N-(dimethoxyphosphoryl)-beta-D-glucopyranosylamine | C8 H18 N O8 P | 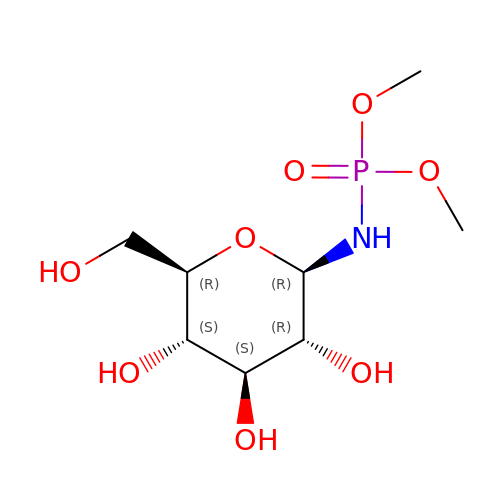LJBUJRWZZYUNKX-JAJWTYFOSA-N NMB0315 is an OMP identified in Neisseria meningitidis as belonging to serogroup B. The development of a universal vaccine against this group remains a challenge. Although few studies have been dedicated to the uncharacterized protein NMB0315, sequence similarities suggest that it is a lysostaphin-type metallopeptidase belonging to the M23 peptidase family. Proteins in this family are characterized by a conserved active site containing an HXH motif, and all are zinc-dependent. Our results suggest that NMB0315 is a zinc-dependent peptidase and belongs to the M23 metallopeptidase family.

The structure of NMB0315 was solved by single-wavelength anomalous dispersion at 2.4 Å resolution. Two molecules of NMB0315 were present in one asymmetric unit. The overall structure consists of three spatially separated domains: Domain I (residues 58–151), Domain II (residues 152–265 and 397–420) and Domain III (residues 266–396). The 2Fo-Fc electron density map reveals a metal ion bound in domain III. This metal ion is coordinated by three spatially adjacent residues (His295, Asp299, and His375) and two water molecules (W142 and W141). Two other histidines, His343 and His373, take part in interactions with the metal ion through the water molecule W141. One possibility is that the Zn2+ was replaced by another metal ion such as Ni2+ during the expression and purification of the protein. In our structure, the short β3-β4 loop of Domain I stretches into the catalytic center of Domain III and forms numerous interactions. Based on these interactions, Domain I of NMB0315 is capable of tightly associating with Domain III, which blocks the active site and the substrate binding groove, suggesting that full-length NMB0315 is in an auto-inhibited conformational state. Based on the comparison of NMB0315 and other M23 metallopeptidases in their active form, we propose that the maturation of NMB0315 requires the amino-terminal domain to be removed.

>GPGSGGSGVQTAYWVQEAVQPGDSLADVLARSGMARDEIARITEKYGGEADLRHLRADQSVHVLVGGDGGAREVQFFTDEDGERNLVALEKKGGIWRRSASEADMKVLPTLRSVVVKTSARGSLARAEVPVEIRESLSGIFAGRFSLDGLKEGDAVRLIYDSLYFHGQQVAAGDILAAEVVKGGTRHQAFYYRSDKEGGGGGNYYDEDGRVLQEKGGFNIEPLVYTRISSPFGYRMHPILHTWRLHTGIDYAAPQGTPVRASADGVITFKGRKGGYGNAVMIRHANGVETLYAHLSAFSQAQGNVRGGEVIGFVGSTGRSTGPHLHYEARINGQPVNPVSVALPTPELTQADKAAFAAQKQKADALLARLR[2x]1-(biphenyl-4-ylmethyl)-1H-imidazole | C16 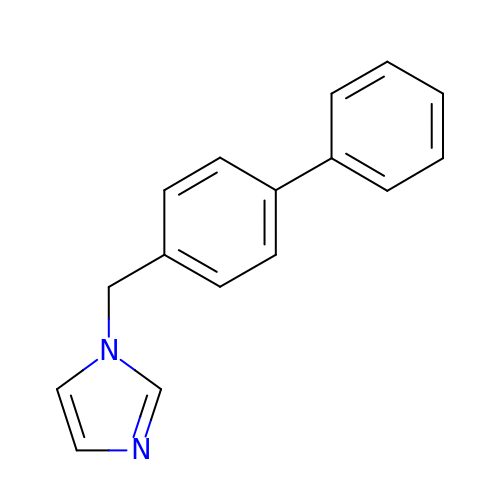H14 N2 | DLYMRVCQTVOYEW-UHFFFAOYSA-N> GVSIRSMKNFYDWIKEFVRDQGEFIAQQSGWLELERSSYAKLIAQTISHVLNGGSLLVSADSSRHWFLNYILSNLNPKDLKERPL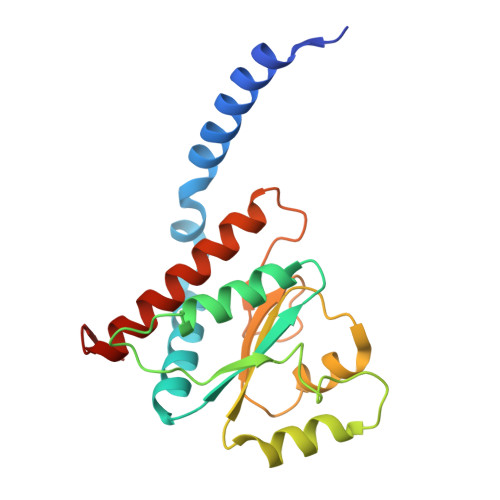LSVIDFNASSFYPKNDANLSLATIEMTYQNPMFWHVGKIENEGLKTILLSKIPSFLWLFEELKEDCLLLKEHDSLLDYKLLQLFKLFENALFSVLYNKVTL> GSHMAGLPRRIIKETQRLLAEPVPGIKAEPDESNARYFHVVIAGPQDSPFEGGTFKLELFLPEEYPMAAPKVRFMTKIYHPNVDKLGRICLDILKDKWSPALQIRTVLLSIQALL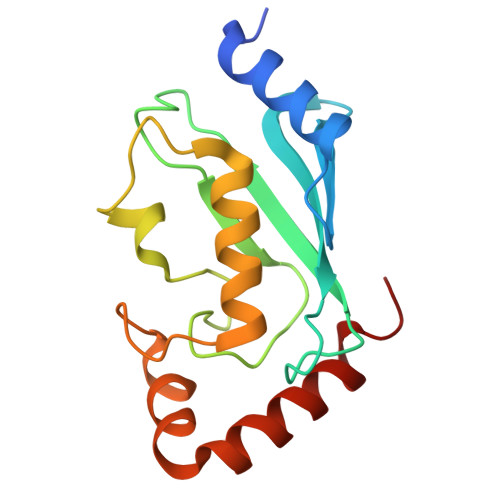SAPNPDDPLANDVAEQWKTNEAQAIETARAWTRLYAMNNI We present here the results of a detailed functional characterization and 3D structure analysis of these three T. melanosporum enzymes, designated as TmelEST 1, 2 and 3, which are shown to be non-lypolitic HSL carboxylesterases closely resembling archaeal and endosymbiotic soil bacteria esterases. The 3D structure of TmelEST2 shows an α/β-hydrolase-fold with well discernible cap and catalytic domains. The latter contains the core region with the catalytic Ser-His-Asp triad, while the less conserved and more dynamic cap domain controls access to the active site and thus likely determines substrate selectivity. The active site of TmelEST2 comprises the Ser190 nucleophile located within the conserved Gly-X-Ser-X-Gly motif, the proton carrier His317 (β7) and the other charge-relay network residue Asp287 (β8).

Because of its superior enzymatic activity and stability, TmelEST2 was selected for crystallization and X-ray diffraction analysis. TmelEST2 crystals (hexagonal space group P6522) contained four protein molecules per asymmetric unit (numbered from A to D), with r.m.s.d. values between Cα atoms of different monomer pairs (referred to monomer A) ranging from 0.18 Å for molecule B to 0.22 Å and 0.29 Å for molecules D and C. The higher r.m.s.d. values for monomers C and D are due to the presence of a Triton-X100 molecule derived from the crystallization medium. Although the structures of the four monomers are largely superimposable (see below), the details of the TmelEST2 structure, which was solved at 2.14 Å resolution, are specifically referred to the detergent-free, monomer A molecule. The four TmelEST2 monomers in the asymmetric unit are arranged as two dimers (A-C and B-D) related by a two-fold axis, one of which (A-C pair) has been used as reference for dimer organization analysis. The substrate-binding pocket is composed of two differently sized, tunnel-shaped cavities (overall volume ~1930Å3), extending from Ser190 to the outer surface of the protein. The Triton X-100 molecule present in monomers C and D is oriented toward the bottom of the substrate-binding pocket, with its aromatic moiety facing a hydrophobic patch within the major substrate-binding pocket close to Ile244 and Ile289 and to the oxyanion-hole, and the hydrophilic polyethylene oxide chain pointing toward the solvent. The detergent-containing monomer exhibits a closer conformation of the substrate entry site, with the loop regions interposed between residues 48–50 and 56–60 shifted by ~1.7 Å toward the Triton-X100 molecule. Indeed, docking analyses conducted on TmelEST2 confirmed the binding of the short acyl-chains of pNPA and pNPB into the very interior of the acyl-binding pocket, whereas the opposite orientation (i.e., with the pNP group pointing inward) was predicted for pNP-octanoate.

>MRFTILSVLAFSLPLVLAETPAPSCPVTNVTTPQLDPITQAYADAISSRPSLFAFPLPEIRDGYQSNVSDPSTEFTTKILSLPVGPTGNVTAYLYKPVSGEREKGKDLLPVIAYFHGGGWVFGGPKSYRGLITNLIRESGAAVFFVDYTLTPKVAYPVPNEQCYAAVQWLLEHGEKLGVDPTNMGFGGDSAGGELSSSVSLLSIKRKTPLPKFQVLIYPATDLACESATFKEFPNGPGLTTDEIRFAASLFTPDPKSRLEDVASPGRASDEDLAKFPETLIVVAEVDPIRQQGEDFGRRLQKLGVRAAIIRVLGTIHGFASIDVLSEAPGAKATIELIGYKFKKALH[4x]>SNAMTKPMIQIALDQTNLTDAVAVASNVASYVDVIEVGTILAFAEGMKAVSTLRHNHPNHILVCDMKTTDGGAILSRMAFEAGADWITVSAAAHIATIAACKKVADELNGEIQIEIYGNWTMQDAKAWVDLGITQAIYHRSRDAELAG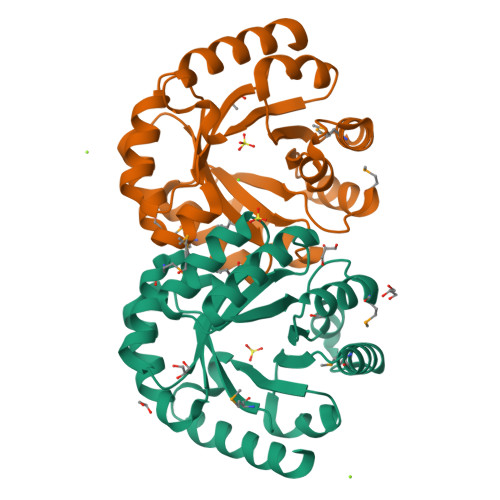IGWTTDDLDKMRQLSALGIELSITGGIVPEDIYLFEGIKTKTFIAGRALAGAEGQQTAAALREQIDRFWP[4x]> GPHMKNVDVEFSQAISYVNKIKTRFADQPDIYKHFLEILQTYQREQKPINEVYAQVTHLFQNAPDLLEDFKKFLPD;> GPRSRLLLGPNSASSSTKLDDDLGTA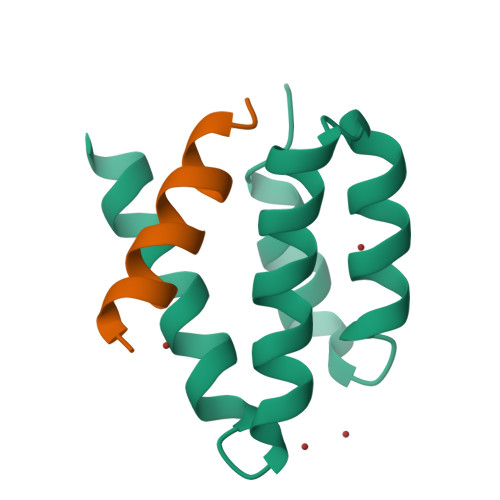AAVLSNMRSSPYRTHDKPIS> GHMSEEQVAQDTEEVFRSYVFYRHQQEQEAEGVAAPADPEMV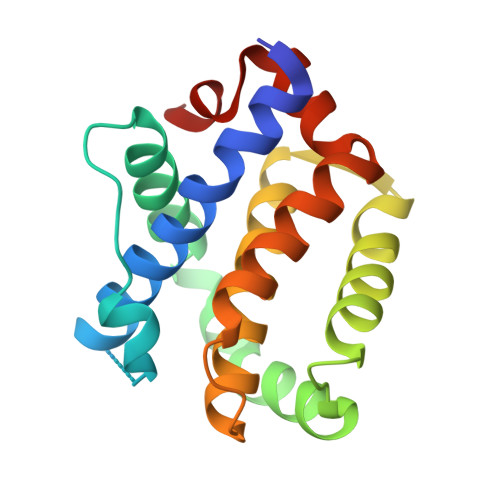TLPLQPSSTMGQVGRQLAIIGDDINRRYDSEFQTMLQHLQPTAENAYEYFTKIATSLFESGINWGRVVALLGFGYRLALHVYQHGLTGFLGQVTRFVVDFMLHHSIARWIAQRGGWVAALNLGN> MALLWQLARNAEGDDPTNLES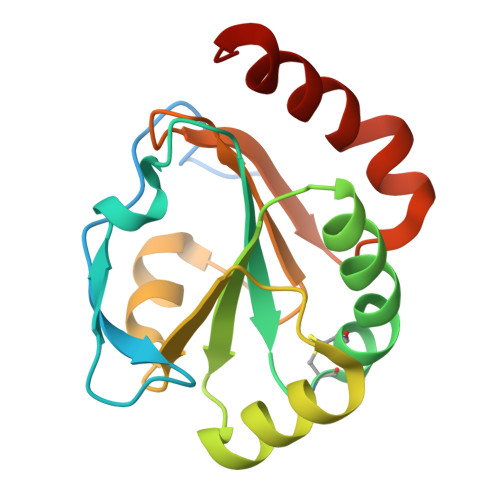ALIGKPVPKFRLESLDNPGQFYQADVLTQGKPVLLNVWATWCPTCRAEHQYLNQLSAQGIRVVGMNYKDDRQKAISWLKELGNPYALSLFDGDGMLGLDLGVYGAAETFLIDGNGIIRYRHAGDLNPRVWEEEIKPLWEKYSKEAAQ> DSRGCARWCPQDSSCVNATACRCNPGFSSFSEIITTPMETCDDINECATLSKVSCGKFSDCWNTEGSYDCVCSPG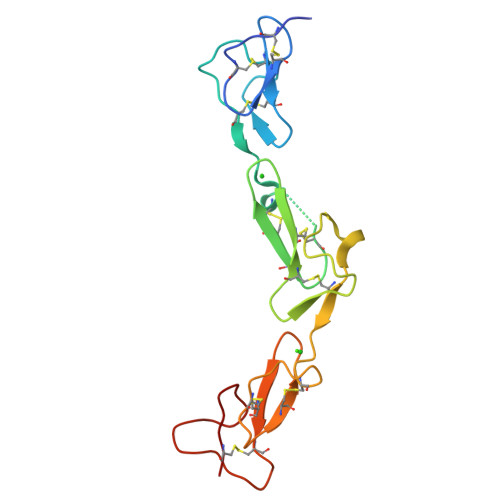YEPVSGAKTFKNESENTCQDVDECSSGQHQCDSSTVCFNTVGSYSCRCRPGWKPRHGIPNNQKDTVCE>GPHMPEKLEAILIPDQGYHQVGPADLCTDMFVLSVTVAFPTKLEQLVPSTMKLSAEGSEFFFYYSLLGNDITSEPFHNLLSPDFEPERASVRIRSSKQILKAFLSQQPSLQIHLCCGNHSLGSTDVSLSALAGISTDLDNKAATVESAFILQPPKRVKQTLPA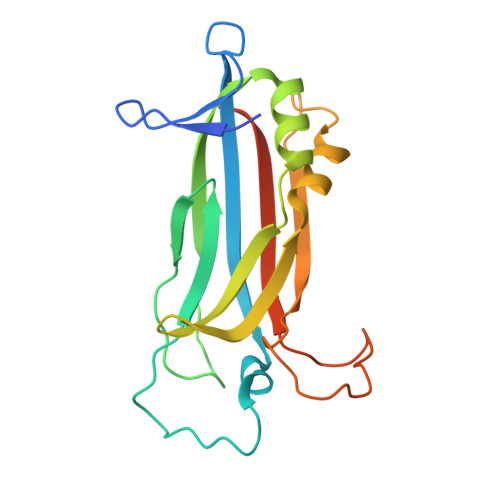LPTDLQPTLGVAVTLRREEVALQQSVGNKE[2x]>MEFTEFNLNELIREVYVLFEEKIRKMNIDFCFETDNEDLRVEADRTRIKQVLINLVQNAIEATGENGKIKITSEDMYTKVRVSVWNSGPPIPEELKEKIFSPFFTTKTQGTGLGLSICRKIIEDEHG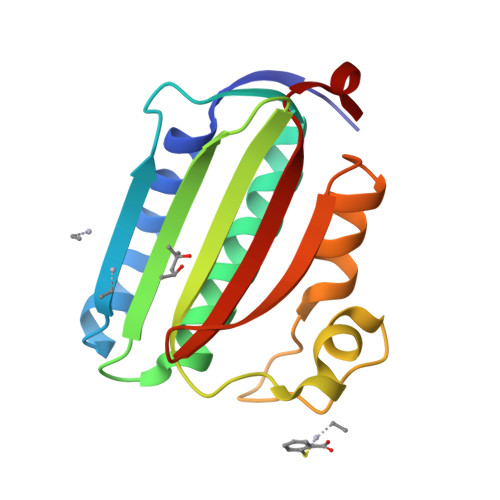GKIWTENRENGVVFIFEIPKTPEKR[2x]>MTTATAGLAVELKQSTAQAHEKAEHSTFMSDLLKGRLGVAEFTRLQEQAWLFYTALEQAVDAVRASGFAESLLDPALNRAEVLARDLDKLNGSSEWRSRITASPAVIDYVNRLEEIRDNVDGPALVAHHYVRYLGDLSGGQVIARMMQRH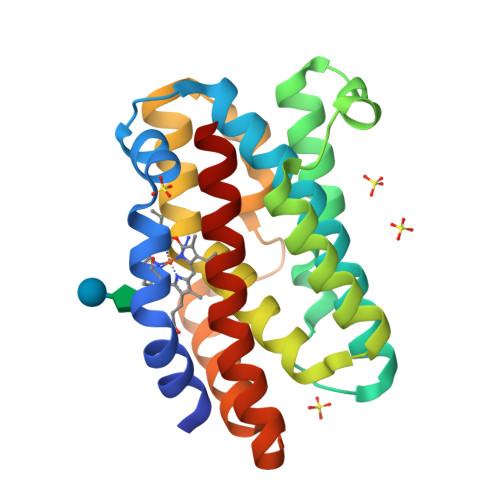YGVDPEALGFYHFEGIAKLKVYKDEYREKLNNLELSDEQREHLLKEATDAFVFNHQVFADLGKGL[2x]> LVKVPLVRKKSLRQNLIKDGKLKDFLKTHKHNPASKYFPEAAALIGDEP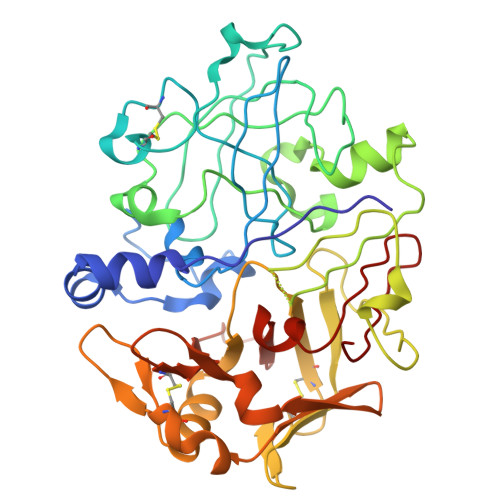LENYLDTEYFGTIGIGTPAQDFTVIFDTGSSNLWVPSVYCSSLACSDHNQFNPDDSSTFEATSQELSITYGTGSMTGILGYDTVQVGGISDTNQIFGLSETEPGSFLYYAPFDGILGLAYPSISASGATPVFDNLWDQGLVSQDLFSVYLSSNDDSGSVVLLGGIDSSYYTGSLNWVPVSVEGYWQITLDSITMDGETIACSGGCQAIVDTGTSLLTGPTSAIANIQSDIGASENSDGEMVISCSSIDSLPDIVFTIDGVQYPLSPSAYILQDDDSCTSGFEGMDVPTSSGELWILGDVFIRQYYTVFDRANNKVGLAPVA> METELSPNLP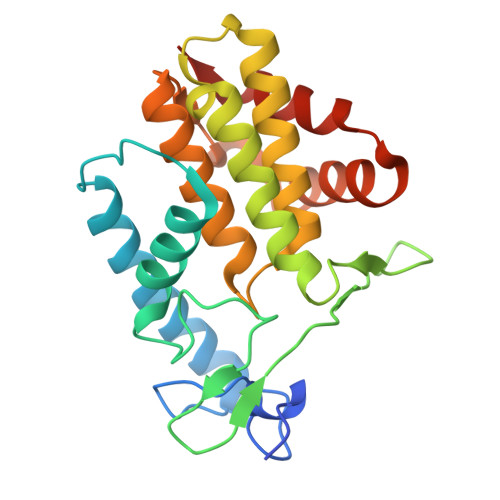LPIYYTYPNSLTLKNKYGIIDHKEFTDKCAHDSAKATINLHQEALPKEFNSSYLKYLHKCLFENTFEWAGCTRDIPFPFKDGTVAVMPEMMRSNWKTDQPIIFAIGNKVQDGLKNIDRILVEKNNLQNLPRQEFIHHLAEIFASLNYTHPFREGNGRTQRIFCEKLAQAANYNLDFSIVTKERMSEVSIAAAQDGNLEPMKKLFDDISHHHHHH BIS(ADENOSINE)-5'-TETRAPHOSPHATE | C20 H28 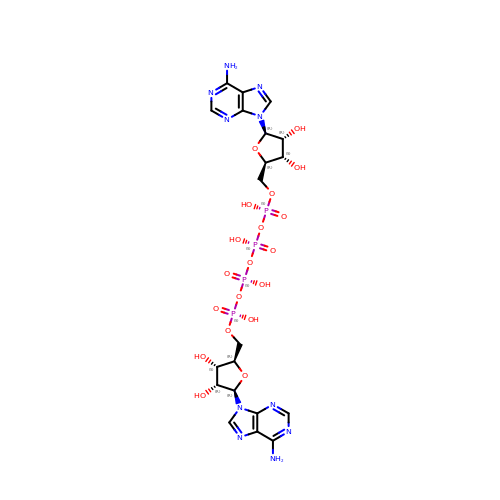N10 O19 P4 | YOAHKNVSNCMZGQ-XPWFQUROSA-N>[2x]SAPRIMRLVAECSRSRARAGELWLPHGTVATPVFMPVGTQATMKGITTEQLDALGCRICLGNTYHLGLRPGPELIQKANGLHGFMNWPHNLLTDSGGFQMVSLVSLSEVTEEGVRFRSPYDGNETLLSPEKSVQIQNALGSDIIMQLDDVVSSTVTGPRVEEAMYRSIRWLDRCIAAHQRPDKQNLFAIIQGGLDADLRATCLEEMTKRDVPGFAIGGLSGGESKSQFWRMVALSTSRLPKDKPRYLMGVGYATDLVVCVALGCDMFDCVFPTRTARFGSALVPTGNLQLRKKVFEKDFGPIDPECTCPTCQKHSRAFLHALLHSDNTAALHHLTVHNIAYQLQLMSAVRTSIVEKRFPDFVRDFMGAMYGDPTLCPTWATDALASVGITLG

In contrast to the homodimeric architecture of the bacterial and archeal TGT, the eukaryotic, heterodimeric TGT is composed of a catalytically active queuine tRNA-ribosyltransferase subunit 1 (QTRT1) and a catalytically inactive QTRT2 subunit. Here we report the first crystal structure of the human QTRT1, which is the catalytic subunit of a eukaryotic TGT enzyme. Analysis of the human QTRT1 catalytic subunit reveals the enzyme to possess a bended (α/β) barrel, consisting of an eight stranded β-barrel at the core and eight flanking helices. In addition, the protein contains a Zn2+ binding domain, in which the zinc ion is coordinated by a triangular arrangement of three cysteine residues Cys317, Cys319, and Cys322, while the α-helix bound His248 completes the tetragonal coordination of the metal ion.

Furthermore, we were able to obtain the structure of human QTRT1 in complex with queuine. Therefore, we chose to soak the ligand into apo crystals. As a consequence of soaking, we did observe additional electron density corresponding to queuine in the active site, that clearly is absent in the apo QTRT1 structure. In addition, the excess electron density map localizes at the site which is equivalent to the preQ1 binding site in the bacterial TGT enzyme. The 7-deaza-guanine moiety is stacking between Phe109 and Met 259 side chains which have previously been implicated in queuine binding in eukaryotic TGTs. Furthermore, correct positioning of the queuine base for the enzymatic reaction is largely provided through polar contacts formed with Asp159. The exocyclic oxygen forms contacts with the polypeptide mainchain at residue Gly229, thus completing the coordination of the 7-deaza-purine. We also did observe density in the mFo-DFc omit map for the additional cyclopentene-cis-diol, a hallmark of this modification, which distinguishes queuine from the bacTGT substrate preQ1. The di-hydroxy-cyclopentene moiety is located in a grove of the protein surface, distant from the QTRT1 catalytic residues and thus also to the anticipated binding site of the RNA substrate. While the space to accommodate the cyclopentene ring is provided by the Gly232 and Gly233 residues, its coordination is achieved by polar contacts of the cyclopentene C5 hydroxy group and Ser164 of the protein chain.> 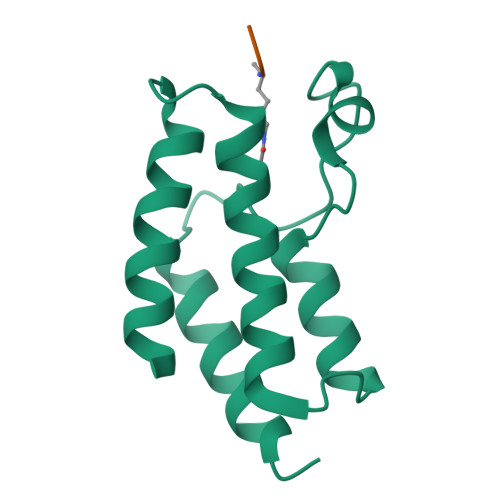GSAENESTPIQQLLEHFLRQLQRKDPHGFFAFPVTDAIAPGYSMIIKHPMDFGTMKDKIVANEYKSVTEFKADFKLMCDNAMTYNRPDTVYYKLAKKILHAGFKMMSK;> SGRGXGGXGLG>MRGSHHHHHHGSSEPLILDAPNADACIIWLHGLGADRTDFKPVAEALQMVLPSTRFILPQAPSQAVTVNGGWVMPSWYDILAFSPARAIDEDQLNASADQVIALIDEQRAKGIAAERIILAGFSQGGAVVLHTAFRRYAQPLGGVLALSTYAPTFDDLALDERHKRIPVLHLH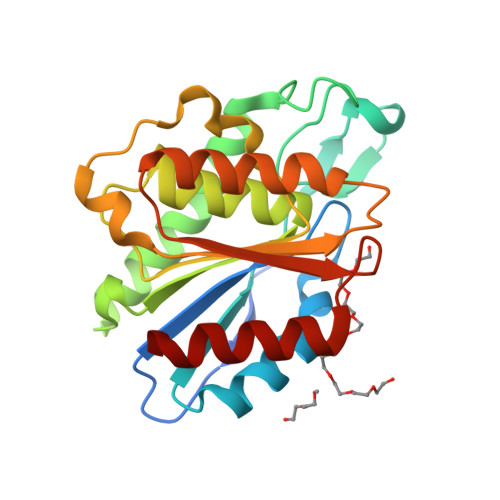GSQDDVVDPALGRAAHDALQAQGVEVGWHDYPMGHEVSLEEIHDIGAWLRKRL[2x]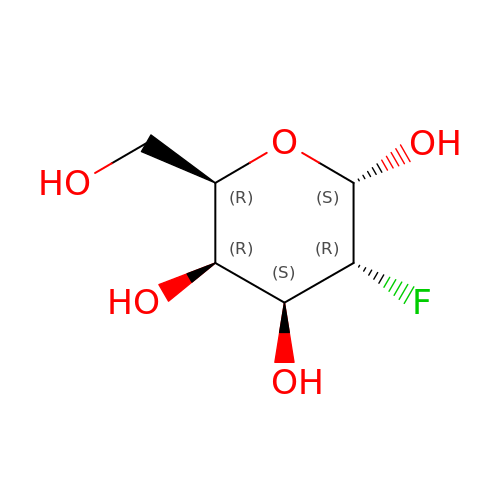2-deoxy-2-fluoro-alpha-D-galactopyranose | C6 H11 F O5 | ZCXUVYAZINUVJD-DVKNGEFBSA-N> SNAMSSAQFDHVTVIKKSNVYFGGLCISHTVQFEDGTKKT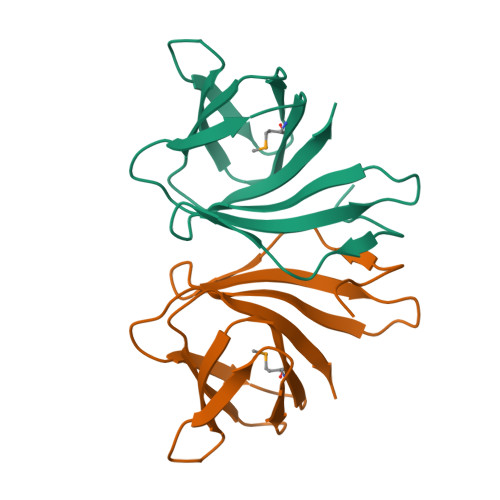LGVILPTEQPLTFETHVPERMEIISGECRVKIADSTESELFRAGQSFYVPGNSLFKIETDEVLDYVCHLEG> HHHHHHDPNEAVREFAKEIDVSFVKIEEVIGAGEFGEVYKGRLKLPGKREIYVAIKTLKAGYSEKQRRDFLSEASIMGQFDHPNIIRLEGVVTKSRPVMIITEFMENGALDSFLRQNDGQFTVIQLVGMLRGIAAGMKYLAEMNYVHRDLAARNILVNSNLVCKVSDFGLSRYLQDDTSDPTYTSSLGGKIPVRWTAPEAIAYRKFTSASDVWSYGIVMWEVMSFGERPYWDMSNQDVINAIEQDYRLPPPMDCPAALHQLMLDCWQKDRNSR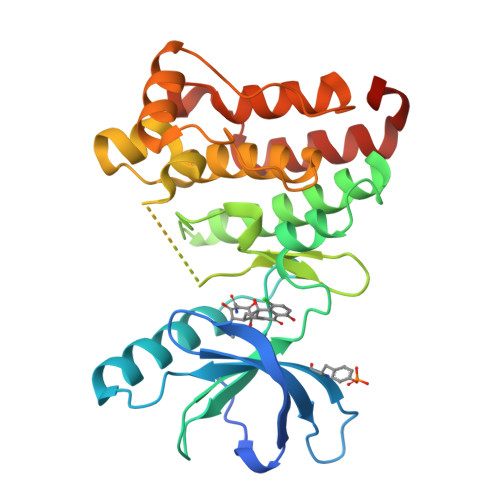PRFAEIVNTLDKMIRNPASLKTVATITA>[2x]MAKGTKYVSKVPDEHGFIEWSTEENLIWQELFTRQIACIKDKACDEYHEGLAKLNLPTDRIPQLDEVSKVLKVSTGWECYPVPALIGFGEFFRLLSEKKFPVATFIR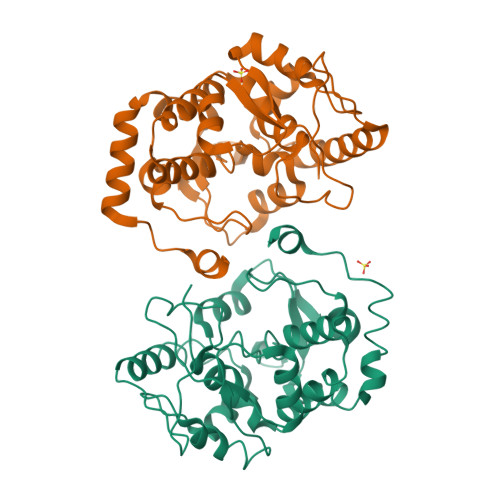SREEMDYLQEPDIFHEIFGHCPLLTNSSFANYTEAYGKMGLNATKEQRVFLARLYWFTIEFGLLDTPKGLRIYGGGVLSSPGETDYAMNNTDVDRKPFDILDVLRTPYRIDIMQPIYYMLTKVSDLDEIRKFEVDDIMELVAQAEALGLHEAKFPVKKAS>PGSIPLIGERFPEMEVTTDHGVIKLPDHYVSQGKWFVLFSHPADFTPVCTTEFVSFARRYEDFQRLGVDLIGLSVDSVFSHIKWKEWIERHIGVRIPFPIIADPQGTVARRLGLLHAESATHTVRGVFIVDA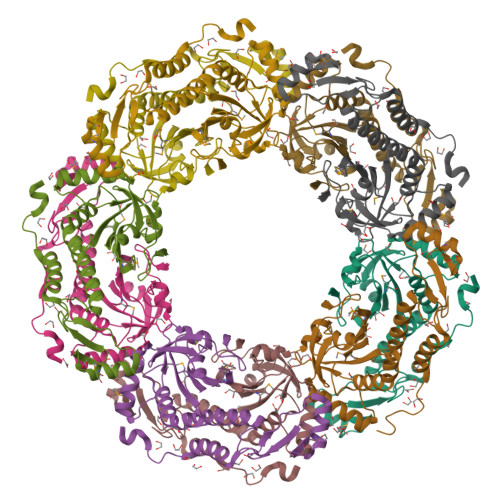RGVIRTMLYYPMELGRLVDEILRIVKALKLGDSLKRAVPADWPNNEIIGEGLIVPPPTTEDQARARMESGQYRSLDWWFCWDTPASRDDVEEARRYLRRAAEKPAKLLYEEARTHLH[10x]>MDINVVNA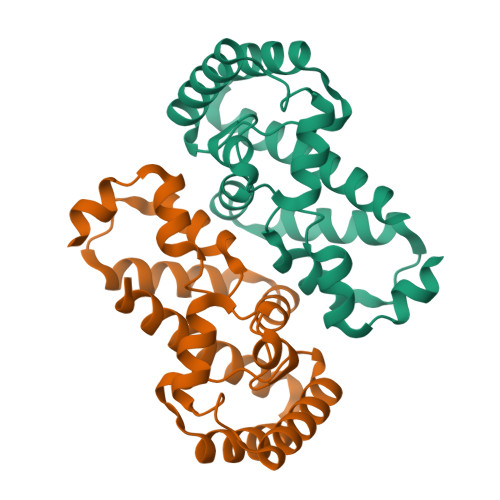LAYEDFVKLFGNVVEKCPLISAAIWSYRPFKDLADIEARISEFIHSLPDSGKEGILRCHPDLAGRDLQSGTLTPESQEEQSQAGMTTLDSAEIVHMYRLNSEYKERFGFPFVICARLNNKADIVRQLSERLKNRRTAELECAIEEVKKICSLRLHSIVLSDIQTKL[6x]> LAHSKMVPIPAGVFTMGTDDPQIKQDGEAPARRVTIDAFYMDAYEVSNTEFEKFVNSTGYLTEAEKFGDSFVFEGMLSEQVKTNIQQAVAAAPWWLPVKGANWRHPEGPDSTILHRPDHPVLHVSWNDAVAYCTWAGKRLPTEAEWEYSCRGGL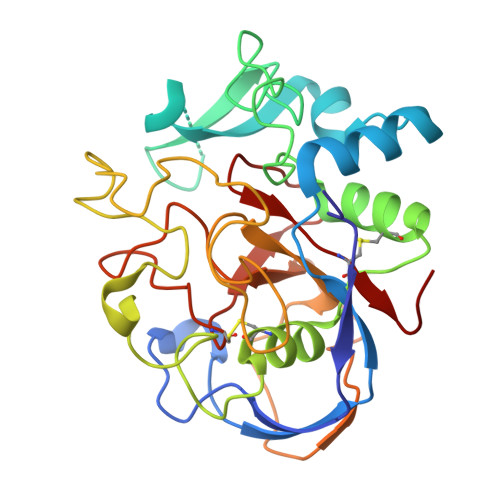HNRLFPWGNKLQPKGQHYANIWQGEFPVTNTGEDGFQGTAPVDAFPPNGYGLYNIVGNAWEWTSDWWTVHHSVEETLNPKGPPSGKDRVKKGGSYMSHRSYCYRYRCAARSQNTPDSSASNLGFRCAADRLP> HPICEVSKVASHLEVNCDKRQLTALPPDLPKDTTILHLSENLLYTFSLATLMPYTRLTQLNLDRCELTKLQVDGTLPVLGTLDLSHNQLQSLPLLGQTLPALTVLDVSFNRLTSLPLGALRGLGELQELYLKGNELKTLPP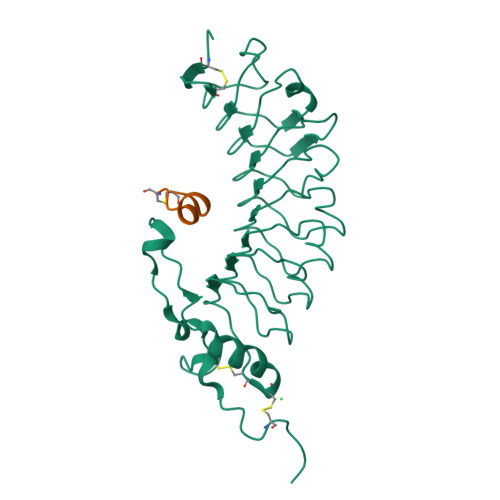GLLTPTPKLEKLSLANNQLTELPAGLLNGLENLDTLLLQENSLYTIPKGFFGSHLLPFAFLHGNPWLCNCEILYFRRWLQDNAENVYVWKQGVDVKAMTSNVASVQCDNSDKFPVYKYPGKGCPLVPR;> CTERMALHNLC>SANSGCKDVTGPDEESFLYFAYGSNLLTERIHLRNPSAAFFCVARLQDFKLDFGNSQGKTSQTWHGGIATIFQSPGDEVWGVVWKMNKSNLNSLDEQEGVKSGMYVVIEVKVATQEGKEITCRSYLMTNYESAPPSPQYKK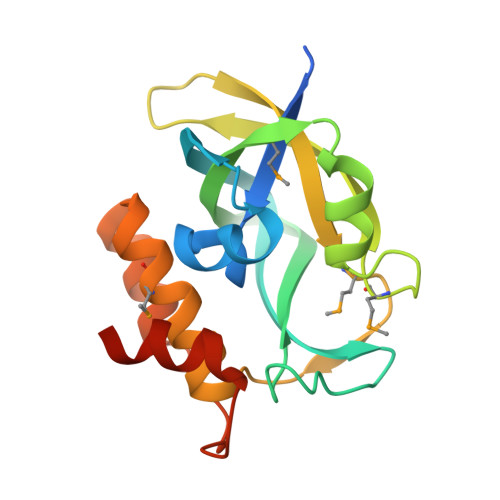IICMGAKENGLPLEYQEKLKAIEPNDYTGKVSEEIEDIIKKGETQTL[2x]> MIERYSREEMSNIWTDQNRYEAWLEVEILACEAWSELGHIPKADVQKIRQNAKVNVERAQEIEQETRHDVVAFTRQVSETLGEERKWVHYGLTSTDVVDTALSFVIKQANDIIEKDLERFIDVLAEKAKNYKYTLMMGRTHGVHAEPTTFGVKMALWYTEMQRNLQRFKQVREEIEVGKMSGAVGTFANIPPEIESYVCKHLGIGTAPVSTQTLQRDRH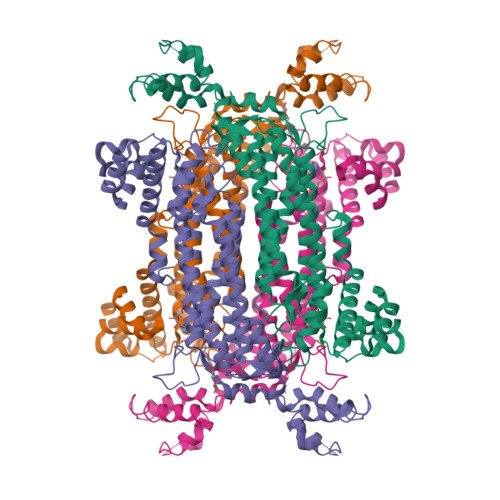AYYIATLALIATSLEKFAVEIRNLQKTETREVEEAFAKGQKGSSAMPHKRNPIGSENITGISRVIRGYITTAYENVPLWHERDISHSSAERIMLPDVTIALDYALNRFTNIVDRLTVFEDNMRNNIDKTFGLIFSQRVLLALINKGMVREEAYDKVQPKAMISWETKTPFRELIEQDESITSVLTKEELDECFDPKHHLNQVDTIFERAGLA> MTSFEDAD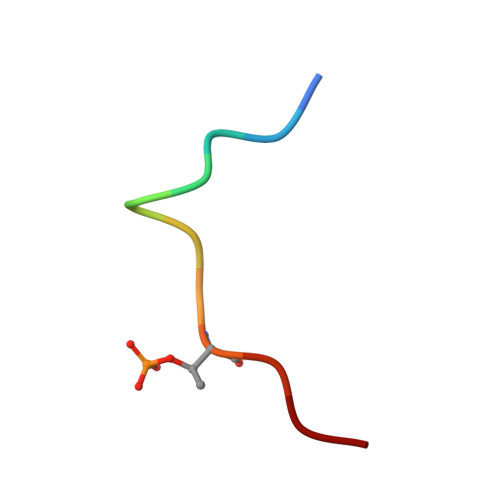TEET>MQGVNIYNISAGTSVDLAAPVTTGDIVTFFSSALNLNAGAGNPNNTTLNLFAENGAYLLHIAFRLQENVIIFNSRQPDGPWLVEQRVSDVANQGAGIDGKAMVTVFDHGDKYQVVINEKTVIQYTKQISGLTSSLSYNATEETSIFSTVVEA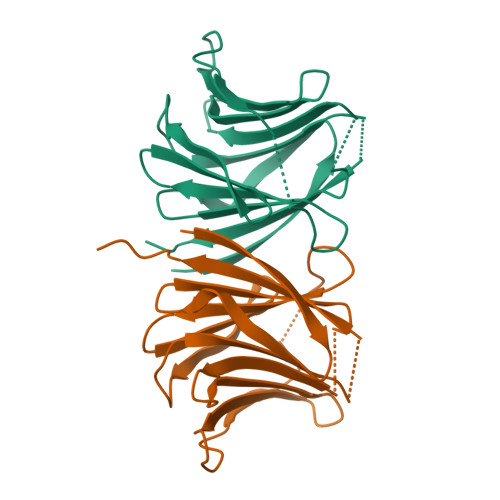VTYTGLALEHHHHHH[2x]> MGMVVALGLDFGASGARAIACDFDSDRSVSVSVTFPKTSQNWPQVWREALWQLLTQIPADWRSRIERIAIDGTSGTVLLCDREGQPQTEPLLYNQACPIDLADLADWVPADHAALSSTSSLAKLWFWQQQFGAL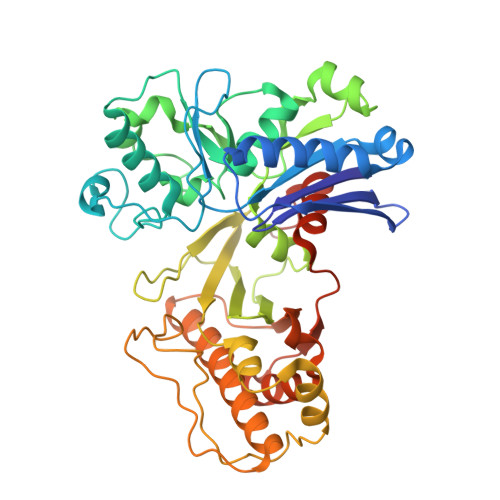PPDWQILAQADWLSLQLHGCSQQSDYHNALKLGYSPDRERFSKNLLDSELGALLPVVHEPGVAIGPILPAIAQEFGLSPDCQICAGTTDSIAAFLASGAHQPGEAVTSLGSTIVLKLLSQVAVSDRLTGVYSHKLGGYWLTGGASNCGGATLRQFFPDTELESLSCQIDPTKKSGLDYYPLPSRGERFPIADPDRLPQLEPRPENPVQFLQGLLEGLTQVETLGYQRLQDLGATPLKRIWTAGGGAKNAVWQQLRQQAIGVPIAIAPNTEAAFGTARLAAFGLAAFHSAGLKRTLEHHHHHH>[2x]SNAMARKTKQQALETRQHILDVALRLFSQQGVSAT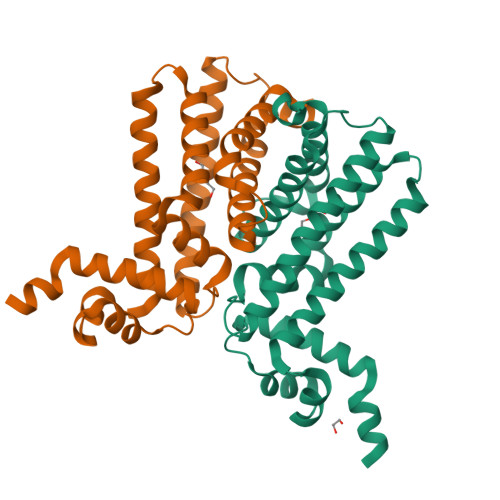SLAEIANAAGVTRGAIYWHFKNKSDLFSEIWELSESNIGELEIEYQAKFPDDPLSVLREILVHILEATVTEERRRLLMEIIFHKCEFVGEMVVVQQAQRSLCLESYDRIEQTLKHCINAKMLPENLLTRRAAILMRSFISGLMENWLFAPQSFDLKKEARAYVTILLEMYQLCPTLRASTVNGSP>TLSLANYLAADSAAEALRRDVRAGLTAAPKSLPPKWFYDAVGSDLFDQITRLPEYYPTRTEAQILRTRSAEIIAAAGADTLVELGSGTSEKTRMLLDAMRDAELLRRFIPFDVDAGVLRSAGAAIGAEYPGIEIDAVCGDFEEHLGKIPHVGRRLVVFLGSTIGNLTPAPRAEF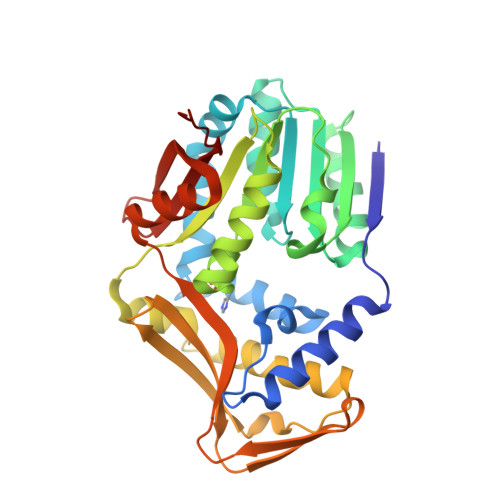LSTLADTLQPGDSLLLGTDLVKDTGRLVRAYDDAAGVTAAFNRNVLAVVNRELSADFDLDAFEHVAKWNSDEERIEMWLRARTAQHVRVAALDLEVDFAAGEEMLTEVSCKFRPENVVAELAEAGLRQTHWWTDPAGDFGLSLAVRLEHHHHHH[2x]> MKRLKKTVASLTAVALLGMGSAAVWAKDIKPRIIRFGYGLADDSPTGKASAHFAEVVSKLSDGKMKVKTFGNGALGPDEQLINSLISGSGEITFVSTAPIASLIPEFGVFDLPFLFDNEKVADTVLDGPEGKKLLDKLPAKGLIGLNYWENGFRNITNSRHEISKLDDIGGIKLRVMQNQVALSVFKGLGANAIPMPFTE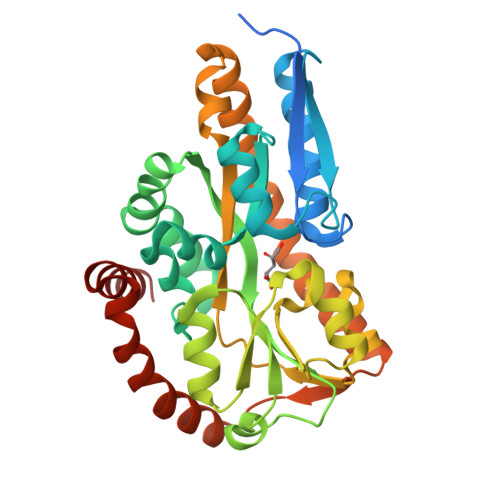LFTALETKTVDGQENPLSTIQTSKFYEVQPYLTLSNHVYTPFVFLASKKWFDQLSQDEKDVITQAAADSQAFQRKASRQGNEDALKYLKEHNVKVAEFSTEEREKIREKVAPIVESLKAKIGKETVEGVLDAAKKASGA>MAHHHHHHMAGTVTESQFKDTM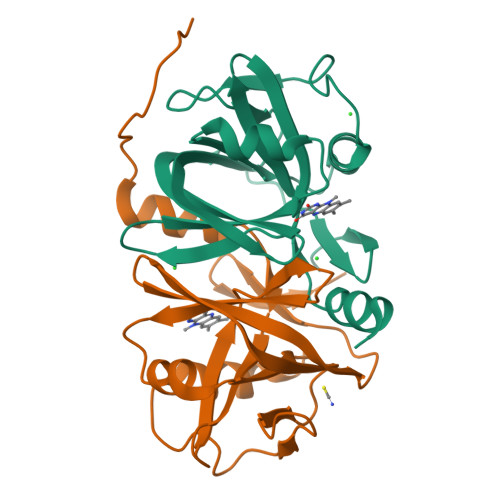SRFPQGVTIITTNCNNELFGFTASSLTSVSLKPPLILFCLNKNSFSINSFQKSDKFAVSILAENQIDISKHFAKSQPNKFTKIAYELGNKTNCPLINGATCYIECNKYASYDAGDHVIFIGEVINTAIKNDLKPLLYFHKSYTNLQ[4x]> MFRGFRPVLAADAVKFQTLYNVLTGKQHLKDQVPVKDCNLTAIFGASWKADLNKWFDSEYAPKLPAAERDSAKK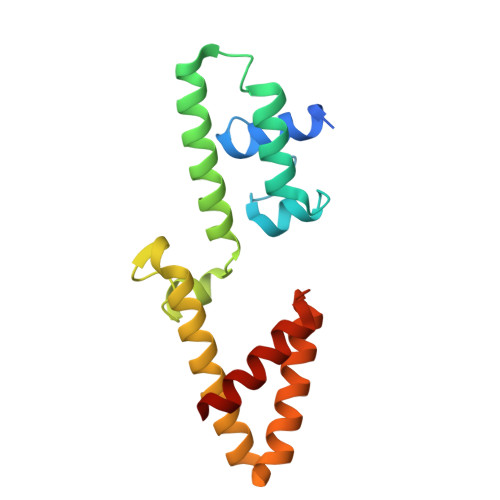SLDLYLKRVDLTRYTREELTTYGILACGPGKVDALTEKHLLETGKARLEELTAGLGNKDEGVNAFRKEVEQEGKYANWPAEKSKALADKVIAASP>[4x]FNLDTEELTAFRVDSAGFGDSVVQYANSWVVVGAPQKITAANQTGGLYQCGYSTGACEPIGLQVPPEAVNMSLGLSLASTTSPSQLLACGPTVHHECGRNMYLTGLCFLLGPTQLTQRLPVSRQECPRQEQDIVFLIDGSGSISSRNFATMMNFVRAVISQFQRPSTQFSLMQFSNKFQTHFTFEEFRRSSNPLSLLASVHQLQGFTYTATAIQNVVHRLFHASYGARRDAAKILIVITDGKKEGDSLDYKDVIPMADAAGIIRYAIGVGLAFQNRNSWKELNDIASKPSQEHIFKVEDFDALKDIQNQLKEKIFAIEGTETTSSSSFELEMAQEGFSAVFTPDGPVLGAVGSFTWSGGAFLYPPNMSPTFINMSQENVDMRDSYLGYSTELALWKGVQSLVLGAPRYQHTGKAVIFTQVSRQWRMKAEVTGTQIGSYFGASLCSVDVDSDGSTDLVLIGAPHYYEQTRGGQVSVCPLPRGWRRWWCDAVLYGEQGHPWGRFGAALTVLGDVNGDKLTDVVIGAPGEEENRGAVYLFHGVLGPSISPSHSQRIAGSQLSSRLQYFGQALSGGQDLTQDGLVDLAVGARGQVLLLRTRPVLWVGVSMQFIPAEIPRSAFECREQVVSEQTLVQSNICLYIDKRSKNLLGSRDLQSSVTLDLALDPGRLSPRATFQETKNRSLSRVRVLGLKAHCENFNLLLPSCVEDSVTPITLRLNFTLVGKPLLAFRNLRPMLAADAQRYFTASLPFEKNCGADHICQDNLGISFSFPGLKSLLVGSNLELNAEVMVWNDGEDSYGTTITFSHPAGLSYRYVAEGQKQGQLRSLHLTCDSAPVGSQGTWSTSCRINHLIFRGGAQITFLATFDVSPKAVLGDRLLLTANVSSENNTPRTSKTTFQLELPVKYAVYTVVSSHEQFTKYLNFSESEEKESHVAMHRYQVNNLGQRDLPVSINFWVPVELNQEAVWMDVEVSHPQNPSLRCSSEKIAPPAS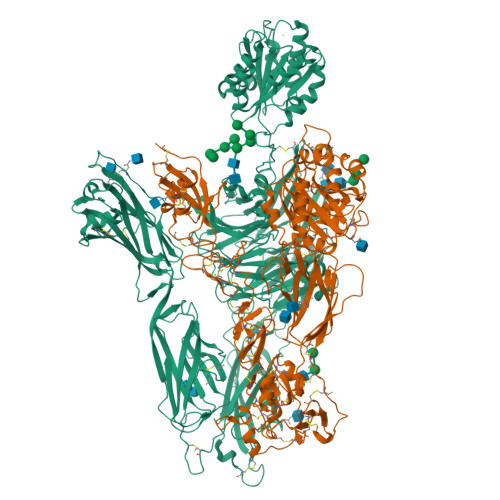DFLAHIQKNPVLDCSIAGCLRFRCDVPSFSVQEELDFTLKGNLSFGWVRQILQKKVSVVSVAEITFDTSVYSQLPGQEAFMRAQTTTVLEKYKVHGCGGLENLYFQGGENAQCEKELQALEKENAQLEWELQALEKELAQWSHPQFEK;>[4x]QECTKFKVSSCRECIESGPGCTWCQKLNFTGPGDPDSIRCDTRPQLLMRGCAADDIMDPTSLAETQEDHNGGQKQLSPQKVTLYLRPGQAAAFNVTFRRAKGYPIDLYYLMDLSYSMLDDLRNVKKLGGDLLRALNEITESGRIGFGSFVDKTVLPFVNTHPDKLRNPCPNKEKECQPPFAFRHVLKLTNNSNQFQTEVGKQLISGNLDAPEGGLDAMMQVAACPEEIGWRNVTRLLVFATDDGFHFAGDGKLGAILTPNDGRCHLEDNLYKRSNEFDYPSVGQLAHKLAENNIQPIFAVTSRMVKTYEKLTEIIPKSAVGELSEDSSNVVQLIKNAYNKLSSRVFLDHNALPDTLKVTYDSFCSNGVTHRNQPRGDCDGVQINVPITFQVKVTATECIQEQSFVIRALGFTDIVTVQVLPQCECRCRDQSRDRSLCHGKGFLECGICRCDTGYIGKNCECQTQGRSSQELEGSCRKDNNSIICSGLGDCVCGQCLCHTSDVPGKLIYGQYCECDTINCERYNGQVCGGPGRGLCFCGKCRCHPGFEGSACQCERTTEGCLNPRRVECSGRGRCRCNVCECHSGYQLPLCQECPGCPSPCGKYISCAECLKFEKGPFGKNCSAACPGLQLSNNPVKGRTCKERDSEGCWVAYTLEQQDGMDRYLIYVDESRECVDGCGLENLYFQGGKNAQCKKKLQALKKKNAQLKWKLQALKKKLAQGGHHHHHH>SDAHHAHKGLNYGSFTKEHVLLTPKGYREWVFIGASVTPNELNDDKAAFPEFHNVYIDPTSWGHWKKTGEFRDGTVIVKELAGVGSKASPSGNGYFPGEFNGIEAMVKDSKRYPERPGNWAFFGFESYEAKQGIIQTDETCAACHKE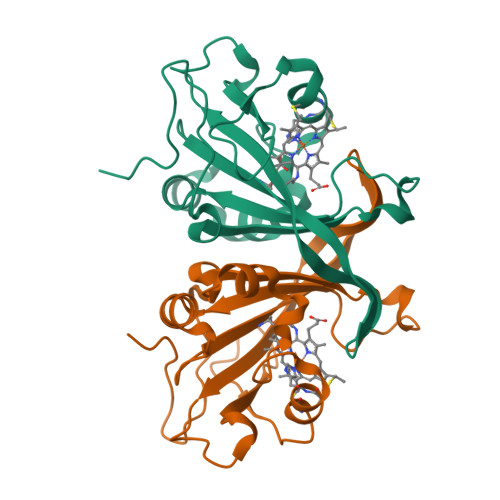HAAHDMVFTQFYPVLRAGKPSK[4x]>[6x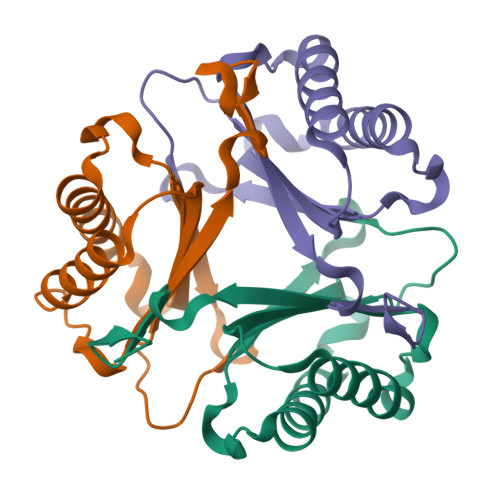]PQLKIYGLREFLDPIKQELSDIINSCMTDALQYPPEKRNQRFFPLERSDFFYPPDRTERYTIIELSMFEGRSVAAKKQLIRLLFERVQPLGISAQDLEITIFETPKHNWGFRGLPGDEH> MRYNQGCQLTAFFIGGNMKIVKHDGYNDIFNGGADGSPKPFFMSDASYHVGSFYNDNATAKRIVDVIPEEMVTAGFKISGVKDEKEFKSLWDSYKIDPSLVDALCWARLYGGAAIVAIINDNRMLTSPVKPGAKLEGVRVYDRFAITIEKRVTNARSPRYGEPEIYKVSPGDNIQPYLIHHTRIFIADG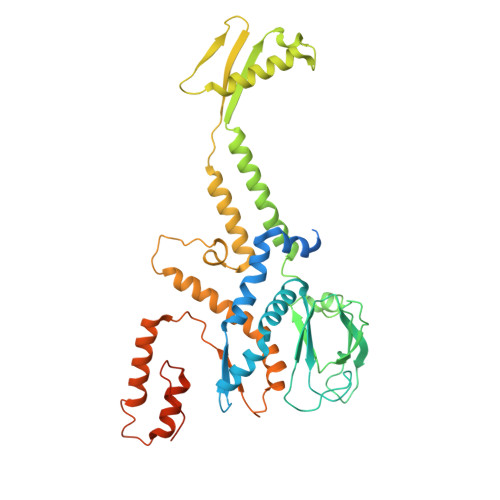ERVTPQMRKQNQGWGASVLNKSLIDAICDYDYCESLATQILRRKQQAVWKVKGLAEMCDDDDAQYAARLRLAQVDDNSGVGRAIGIDAETEEYDVLNSDISGVPEFLSSKMDRIVSLSGIHEIIIKNKNVGGVSASQNTALETFYKLVDRKREEDYRPLLEFLLPFIVDEQEWSIEFEPLSVPSKKEESEITKNNVESVTKAITEQIIDLEEARDTLRSIAPEFKLKDGNNINIREPEEPTEPEPGLGEKLEDEN> MNSSIKKIYNHIQEKVINYSDTIDLADGNYVVSRGDGWILSRQNQILGGSVISNGSTGIVGDLRVNDNAIPYYYPTPSFNEEYIKNNIQTVFANFTEANQIPIGFEFSKTAPSNKNLYMYLQYTYIRYEIIKVLQHEIIERAVLYVPSLGYVKSIEFNPGEKINKDFYFLTNDKCILNEQFLYKKILETTKNIPTNNIFNSKVSSTQRVLPYSNGLYVINKGDGYIRTNDKDLIGTLLIEAGSSGSIIQPRLRNTTRPLFTTSNDAKFSQQYTEERLKDAFNVQLFNTSTSLFKFVEEAPSNKNICIKAYNTYEKYELIDYQNGSIVNKAEYYLPSLGYCEVTNAPSPESEVVKTQVAEDGFIQNGPEEEIVVGVIDPSENIQEINTAISDNYTYNIPGIVNNNPFYILFTVNTTGIYKINAQNNLPSLKIYEAIGSGNRNFQSGNLCDDDIKAINYITGFDSPNAKSYLVVLLNKDKNYYIRVPQTSSNIENQIKFKREEGDLRNLMNSSVNIIDNLNSTGAHYYTRQSPDVHDYISY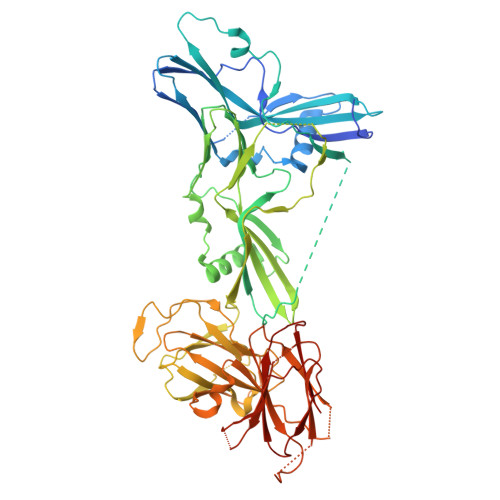EFTIPGNFNNKDTSNIRLYTSYNQGIGTLFRVTETIDGYNLINIQQNLNLLNSTKSIRLLNGAIYILKVEVTELNNYNIKLHIDITN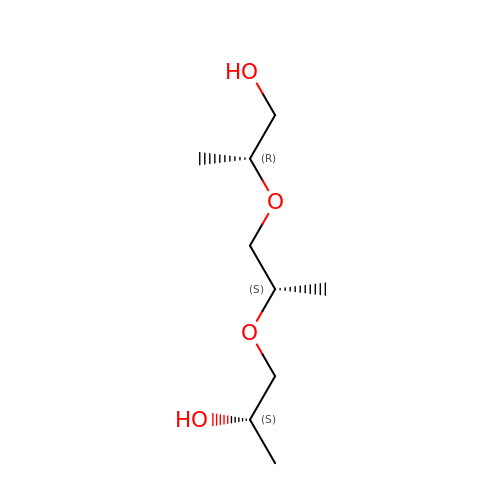(2R)-2-[(2S)-2-[(2S)-2-oxidanylpropoxy]propoxy]propan-1-ol | C9 H20 O4 | LCZVSXRMYJUNFX-YIZRAAEISA-N ethyl 5-nitrothiophene-2-carboxylate | C7 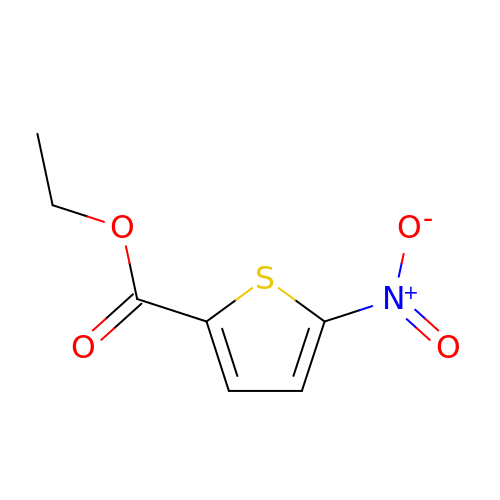H7 N O4 S | COLIROLDWDCDLN-UHFFFAOYSA-N> MATKLDYEDAVFYFVDDDKICSRDSIIDLIDEYITWRNHVIVFNKDITSCGRLYKELMKFDDVAIRYYGIDKINEIVEAMSEGDHYINFTKVHDQESLFATIGICAKITEHWGYKKISESRFQSLGNITDLMTDDNINILILF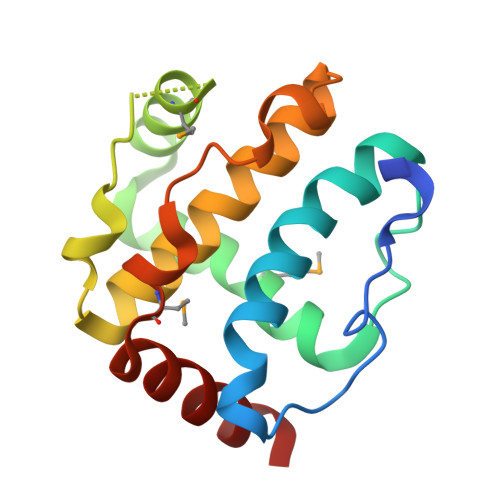LEKKLN>MATAQSNSPRVFCIGTADTKFDELRFLSEHVRSSLNSFSNKSSFKVGVTVVDVSTSWKETNSCADFDFVPSKDVLSCHTLGEETMGTFADTRGLAIAIMSKALETFLSIANDEQNLAGVIGLGGSGGTSLLSSAF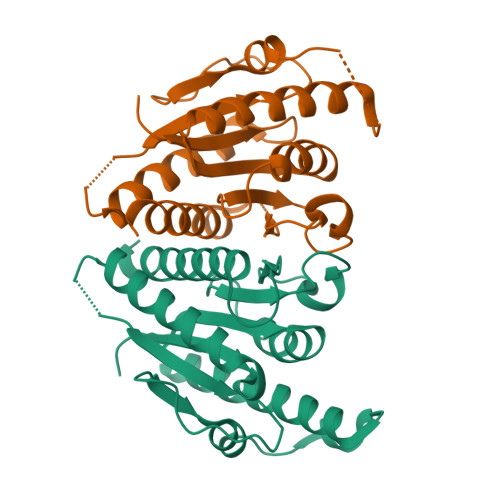RSLPIGIPKVIISTVASGQTESYIGTSDLVLFPSVVDICGINNVSKVVLSNAGAAFAGMVIGRLES[2x]>[2x]GSHMVNMVSNPGFEDGLDSWQDWQQDMSAVPEAAHNGALGLKIGGGKAAGGGQDIPLKPNTTYILGAWAKFDSKPAGTFDVVVQYHLKDANNTYVQHILNFNETDWTYKQLL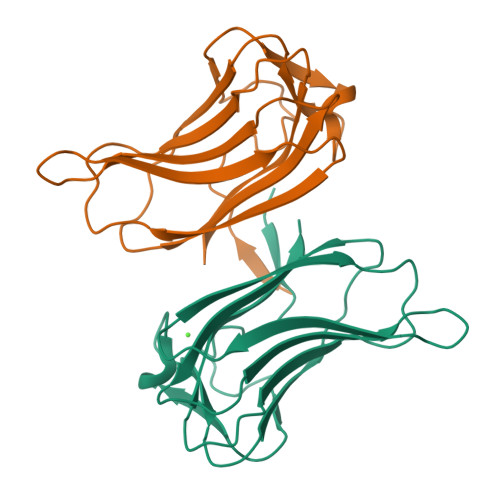FTTPDVFGSTPQLALWKGDTSKANLYVDDVYLVEV> ASSPANKVYQDRFESMYSKIKDPANGYFSEQGIPYHSIETLMVQAPDYGHVTTSEAMSYYMWLEAMHGRFSGD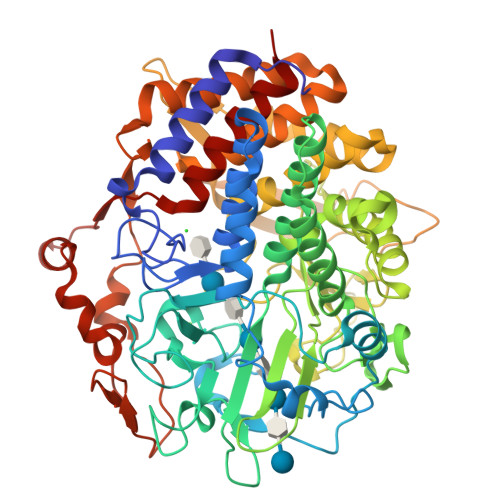FTGFDKSWSVTEQYLIPTEKDQPNTSMSRYDANKPATYAPEFQDPSKYPSPLDTSQPVGRDPINSQLTSAYGTSMLYGMHWILDVDNWYGFGARADGTSKPSYINTFQRGEQESTWETIPQPCWDEHKFGGQYGFLDLFTKDTGTPAKQFKYTNAPDADARAVQATYWADQWAKEQGKSVSTSVGKATKMGDYLRYSFFDKYFRKIGQPSQAGTGYDAAHYLLSWYYAWGGGIDSTWSWIIGSSHNHFGYQNPFAAWVLSTDANFKPKSSNGASDWAKSLDRQLEFYQWLQSAEGAIAGGATNSWNGRYEAVPSGTSTFYGMGYVENPVYADPGSNTWFGMQVWSMQRVAELYYKTGDARAKKLLDKWAKWINGEIKFNADGTFQIPSTIDWEGQPDTWNPTQGYTGNANLHVKVVNYGTDLGCASSLANTLTYYAAKSGDETSRQNAQKLLDAMWNNYSDSKGISTVEQRGDYHRFLDQEVFVPAGWTGKMPNGDVIKSGVKFIDIRSKYKQDPEWQTMVAALQAGQVPTQRLHRFWAQSEFAVANGVYAILFPD>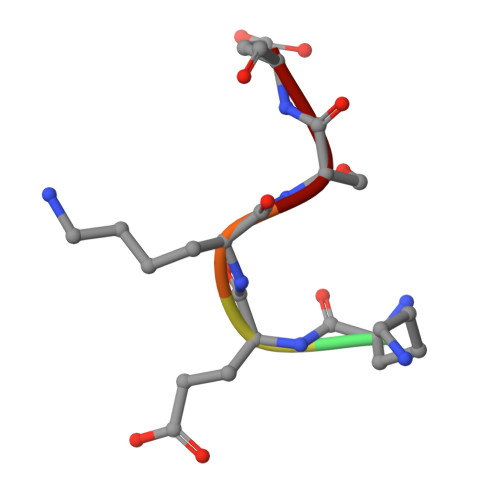 AKEKSD>[2x]NAQFLHTQVGRGLLGAVVNPLGEVTDKFAVTDNSEILYRPVDNAPPLYSERAAIEKPFLTGIKVIDSLLTCGEGQRMGIFASAGCGKTFLMNMLIEHSGADIYVIGLIGEAGAEVTETVDYLKNSEKKSRCVLVYATSDYSSVDRCNAAYIATAIAEFFRTEGHKVALFIDSLTRYARALRDVALAAGESPARRGYPVSVFDSLPRLLERPGKLKAGGSITAFYTVLL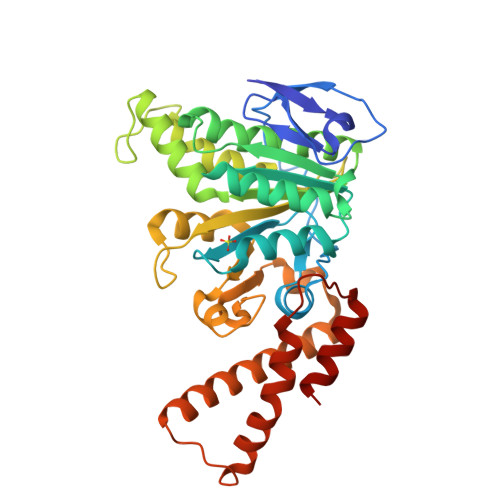EDDDFADPLAEEVRSILDGHIYLSRNLAQKGQFPAIDSLKSISRVFTQVVDEKHRIMAAAFRELLSEIEELRTIIDFGEYKPGENASQDKIYNKISVVESFLKQDYRLGFTYEQTMELIGETIR>[12x]MAKFPKNFMFGYSWSGFQFEMGLPGSEVESDWWVWVHDKENIASGLVSGDLPENGPAYWHLYKQDHDIAEKLGMDCIRGGIEWARIFPKPTFDVKVDVEKDEEGNIISVDVPESTIKELEKIANMEALEHYRKIYSDWKERGKTFILNLYHWPLPLWIHDPIAVRKLGPDAAPAGWLDEKTVVEFVKFAAFVAYHLDDLVDMWSTMNEPNVVYNQGYINLASGFPPGFLSFEAAEKAKFNLIQAHIGAYDAIKEYSEKSVGVIYAFAWHDPLAEEYKDEVEEIRKKDYEFVTILHSKGKLDWIGVNYYSRLVYGAKDGHLVPLPGYGFMSERGGFAKSGRPASDFGWEMYPEGLENLLKYLNNAYELPMIITENGMADAADRYRPHYLVSHLKAVYNAMKEGADVRGYLHWSLTDNYEWAQGFRMRFGLVYVDFETKKRYLRPSALVSVK

One of the β-glucosidases from Pyrococcus furiosus (BGLPf) is found to be a hyperthermophilic tetrameric enzyme that can degrade cellooligosaccharides. Cellulase systems consist of three categories of cellulase that catalyze the conversion of cellulose into glucose: endoglucanases (EGs), cellobiohydrolases (CBHs) and β-glucosidases (BGLs). BGL (BGLPf, family 1) isolated from Pyrococcus furiosus exhibits high hydrolytic activity towards cellooligosaccharides at high temperature. The structure of BGLPf shows a stable homotetrameric structure forming 222 point-group symmetry.

Here, a new monomeric form of BGLPf was constructed by removing the C-terminal region of the enzyme and its crystal structure was solved at a resolution of 2.8 Å in space group P1. The asymmetric unit exhibits a unique duplicated hexameric ring structure that includes the 12 monomers; one of the rings includes six monomers named A, C, E, G, I and K, and the other also includes six monomers named B, D, F, H, J and L. The arrangement of monomers therefore generates a local sixfold symmetrical axis that is not parallel to any of the crystal axes a, b and c, and hence the space group is P1. Analysis of the protein interfaces by PISA did not reveal sufficient interactions that could result in the formation of stable quaternary structures. Thus, the structures of monomers A, B, C, D, E, F, G, H, I, J, K and L are able to form a pseudo-dodecameric structure in the crystal, a complex that is presumably difficult to form in aqueous solution. The deletion of the C-terminal region of BGLPf, which drastically altered the crystal packing into space group P1, did not however affect the individual structures of monomeric BGLPf. Furthermore, the r.m.s. deviations of the Cα-atom positions (2–449) of subunits A, B, C, D, E, F, G, H, I, J, K and L of BGLPf-M6ΔC compared with subunit A of BGLPf-WT were between 0.44 and 0.71 Å, even though the region Asp96–Val108 showed a small mismatch of more than 2 Å. The results indicated that BGLPf-M6ΔC (63 kDa) is monomeric in aqueous solution. The hydrodynamic radius of BGLPf-M6ΔC was estimated to be 3.1 nm. Therefore, the results obtained so far demonstrate that thermostability is not determined by the C-terminal length of BGL, but rather depends on its polymeric state. We successfully constructed a monomeric form of the enzyme by removing its C-terminal region and solved the crystal structure. This study shows that the lack of the C-terminal region does not affect the activity of the enzyme, but disrupts its oligomeric state and hyperthermostability.>[4x]MVTALSDVNNTDNYGAGQIQVLEGLEAARKRPGMYIGSTSERGLHHLV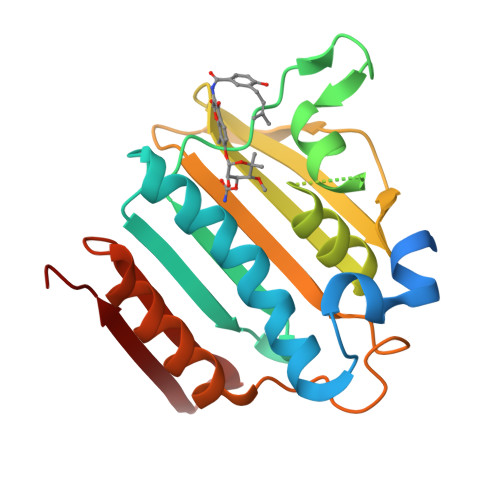WEIVDNSIDEALAGYANQIEVVIEKDNWIKVTDNGRGIPVDIQEKMGRPAVEVILTVLHAGGKFGGGGYKVSGGLHGVGSSVVNALSQDLEVYVHRNETIYHQAYKKGVPQFDLKEVGTTDKTGTVIRFKADGEIFTETTVYNYETLQQRIRELAFLNKGIQITLRDERDEENVREDSYHYEG1-{2-[5-(2-methoxyethoxy)-1H-benzimidazol-1-yl]quinolin-8-yl}piperidin-4-amine | C24 H27 N5 O2 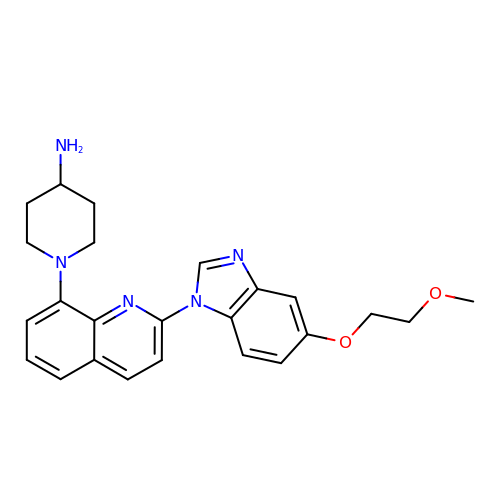| DEEOXSOLTLIWMG-UHFFFAOYSA-N Type III secretion systems (T3SS) allow the transport of protein substrates directly across the double membrane of Gram-negative bacteria. Proteomic analyses have identified the major components of the sorting platform for the Salmonella typhimurium SPI-1 injectisome: the AAA+ ATPase InvC, its regulator OrgB and the proteins SpaO and OrgA4. Here we show that a novel, heterotypic interaction between SPOA domains serves as a scaffold for sorting platform assembly in both injectisome and flagellar T3SS. Our structures suggest a partial model for the subtype-specific assembly of the T3SS sorting platforms: the heterotypic interaction between SPOA domains within a given T3SS subtype functions as an adaptor for ATPase and its regulator through interaction with the APAR peptide.

Preliminary bioinformatic analyses suggested the presence of two putative SPOA domains in the carboxy-terminal half of SpaO, which we denote SPOA1 and SPOA2. We first determined the structure of the SPOA2 homodimer to 1.35 Å resolution. The SPOA2 homodimer structure is architecturally similar to its homologues: like two left hands grasping one another, an antiparallel beta-sheet ‘palm' of each protomer is grasped by the ‘fingers' of the other, with a ‘thumb' protruding from the top of the palm and strands from each protomer forming an antiparallel beta sheet on the ‘floor' of the assembly. The Salmonella SPOA2 homodimer superposes on its Yersinia and Pseudomonas homologues with 2.24 and 3.05 Å root mean squared deviation (r.m.s.d.), respectively. In both SPOA1,2 and the SPOA2 homodimer, interacting protomers each bury about 1,800 Å2 against their binding partner. It should be noted that SpaO(1–219) does not complement a full genomic deletion of spaO, demonstrating that SPOA2 is also necessary for T3SS function. Indeed, SPOA1,2 is sufficient to co-affinity purify OrgB–InvC. This construct contains a Val203GTG-to-Val203GTT mutation to prevent the duplicitous translation of SPOA2 from its cryptic internal translation start site, demonstrating that the SPOA2 homodimer is dispensable for SpaO–OrgB–InvC complex formation.

>GPVDVKLEFVLYRKNVTLAELEAMGQQQLLSLPTNAELNVEIMANGVLLGNGELVQMNDTLGVEIHEWLS[2x]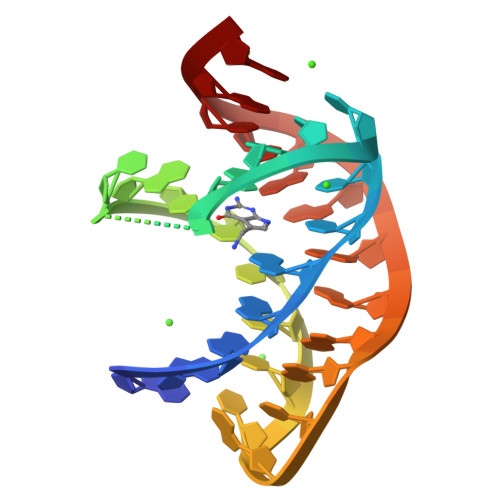>[3x]AGAGGUUCUAGCUACACCCUCUAUAAAAAACUAA>LYQLEN[2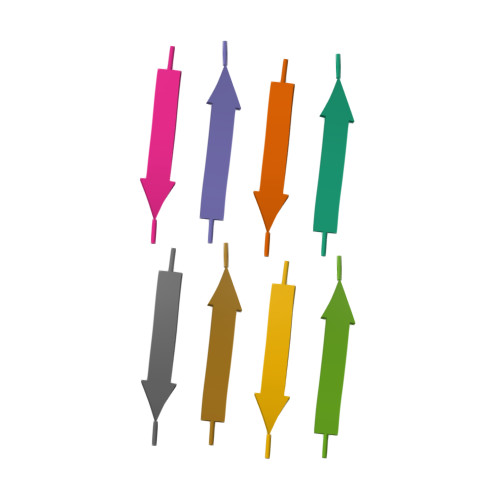x]> PVNLIFCYTILQMKVAERIMAQHPGERFYVVLMSENRNEKYDYYFNQIKDKAEWAYFF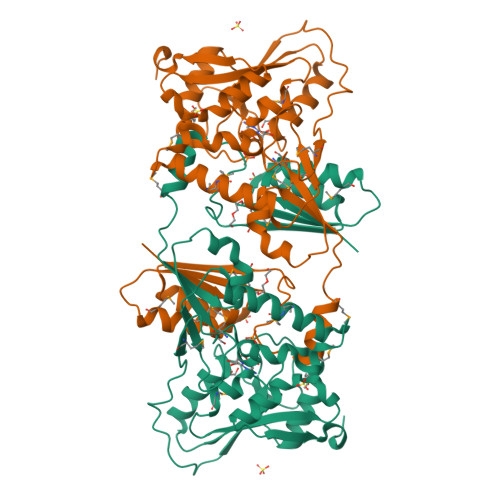HLPYGLNKSFNFIPTMAELKVKAMLLPKVKRIYLASLEKVSIAAFLSTYPDAEIKTFDDGTINLIQSSSYLGDEFSVNGTIKRNFARMMIGDWSIAKTRNASDEHYTIFKGLKNIMDDGRRKMTYLPLFDASELKAGDETGGTVRILLGSPDKEMKEISEKAAKNFNIQYVAPHPRQTYGLSGVTTLNSPYVIEDYILREIKKNPHTRYEIYTFFSGAALTMKDFPNVHVYALKPASLPEDYWLKPVYALFTQSGIPILTFDDKLVPR Nucleotide-binding domain, leucine-rich repeat receptors (NLRs) mediate innate immunity by forming inflammasomes. Activation of the NLR protein NLRP1 requires autocleavage within its function-to-find domain (FIIND). In resting cells, the dipeptidyl peptidases DPP8 and DPP9 interact with the FIIND of NLRP1 and suppress spontaneous NLRP1 activation; however, the mechanisms through which this occurs remain unknown. Here we present structural and biochemical evidence that full-length rat NLRP1 (rNLRP1) and rat DPP9 (rDPP9) form a 2:1 complex that contains an autoinhibited rNLRP1 molecule and an active UPA–CARD fragment of rNLRP1.

Two-dimensional class averages showed that rDPP9 formed dimers, but only one subunit was bound to NLRP1 in most of the particles. We used the particles with one rDPP9 subunit bound by rNLRP1 for further cryo-EM analysis. After 3D classification, a subset of 182,116 particles was used for final 3D reconstruction, generating a map with a global resolution of 3.18 Å. Unexpectedly, the liganded rDPP9 subunit is bound by two rNLRP1 molecules, which we hereafter term the 2:1 rNLRP1–rDPP9 complex. The first rNLRP1 molecule contains the complete FIIND, which has a conformation nearly identical to that observed in the crystal structure of the free FIIND; the remaining domains of this rNLRP1 molecule are not discernible in the cryo-EM density. In the second rNLRP1 molecule, only the UPA domain is well defined. Three surfaces mediate the formation of the 2:1 rNLRP1–rDPP9 complex. The first surface is mediated by ZU5 of rNLRP1, which binds to one lateral side of the β-propeller domain of rDPP9 (termed the ZU5-binding site of rDPP9). The second interface is formed by the deep insertion of an N-terminal loop (N-loop) from the UPA domain of the second rNLRP1 molecule into the rDPP9 substrate-binding channel (termed the UPA-binding site) (blue box). The substrate-binding groove of rDPP9 is completely blocked by the UPA N-loop. Additionally, the homodimerization interface of the two UPA domains also contributes to formation of the 2:1 complex (termed the UPA dimerization site) (yellow box).

>MEESQSKQESNTRVAQHGSQQDVDPTFQTKRALEKERSKPRPRPLPRVQLQSLPGWSSTSKDVPLSQLIREMDHESRRCIHRSKKKLDRSEHISQGTIPEIYEKRKETISHTQSMEQKYLFQNFTKLLLLQKCCPGGSEKLVRESWHPCVPEEGGHMIEIQDLFDPNLDTEKKPQLVIIEGAAGIGKSTLARQVKRAWDEGQLYRDRFQHVFFFSCRELAQCKQLSLAELIAQGQEVPTAPTRQILSRPEKLLFILDGIDEPAWVLEDQNPELCVHWSQAQPVHTLLGSLLGKSILPEASLMLTARTTALQKLVPSLGQPHRVEVLGFSEFERKDYFYKYFAKERNTIIDFNLIGSIPVLLTLCEVPWVCWLLCTCLEKQMQQGEVLSLTSQTTTALCLKYLSLTIPGQHLSTQLRTLCSLAAEGICQRRTLFSKSDLCKQGLAEDAIATFLKIGVLQRQPSSLSYSFAHLCLQEFFAAMSYILEDSEEAHGDMGNDRTVETLVERYGRQNLFEAPTVRFLLGLLNTREMREMENIFACKFPWETKLKLLQSIIGEPFCQPCHLGLFHCLYENQEEELLTETMLCFPLTASGPNHMEATVFQTNVKRLVIQTDMELMVVTFCITFSHVRSLRLKGKGQQEYKLTAPAMVLYRWTPISEASWKVLFSNLKCTRNLEELDLSGNPLSYSAVRSLCTALRQPGCRLKTLWLVDCGLTSRCCSFLASMLSAHSRLAELDLRLNDLGDNGVRQLCEGLRNPACNLSILRLDQASLSEQVITELRALETKNPKLFISSTWMSHMTMPTENTDGEESLTSSKQQQQQSGDKHMEPLGTDDDFWGPSGPVSTEVVDRERNLYRVRLPMAGSYHCPSTGLHFVVTRAVTIEIGFCAWSQFLHETPLQHSHMVAGPLFDIKAEHGAVTAVCLPHFVSLQEGKVDSSLFHVAHFQDHGMVLETPARVEPHFAVLENPSFSPMGVLLRMIPAVGHFIPITSITLIYYRLYLEDITFHLYLVPNDCTIRKAIDEEELKFQFVRINKPPPVDALYVGSRYIVSSSKEVEILPKELELCYRSPRESQLFSEIYVGNIGSGINLQLTDKKYMNLIWEALLKPGDLRPALPRMASAPKDAPALLHFVDQHREQLVARVTSVDPLLDKLHGLVLSEEDYETVRAEATNQDKMRKLFRGSRSWSWDCKDHFYQALKETHPHLIMDLLEKSGGVSVRL[2x];>MSGGVSPVEQVAAGDMDDTAARFCVQKHSWDGLRNIIHGSRKSSGLIVSKAPHDFQFVQKPDESGPHSHRLYYLGMPYGSRENSLLYSEIPKKVRKEALLLLSWKQMLDHFQATPHHGVYSREEELLRERKRLGVFGITSYDFHSESGLFLFQASNSLFHCRDGGKNGFMVSPMKPLEIKTQCSGPRMDPKICPADPAFFSFINNNDLWVANIETGEERRLTFCHQGSASVLDNPKSAGVATFVIQEEFDRFTGCWWCPTASWEGSGGLKTLRILYEEVDESEVEVIHVPSPALEERKTDSYRYPRTGSKNPKIALKLAELQTDHQGKIVSSCEKELVQPFSSLFPKVEYIARAGWTRDGRYAWAMFLDRPQQRLQLVLLPPALFIPTLESEAQWQEAARAIPKNVQPFIIYEEVTNVWINVHDIFHPFPQAEGQQDFCFLRANECKTGFCHLYRVTVDLKTNDYDWTEPLSPAEDEFKCPIKEEVALTSGEWEVLSRHGSKIWVNEQTKLVYFQGTKDTPLEHHLYVVSYESAGEIVRLTTPGFSHSCSMSQNFDMFVSHYSSVSTPPCVHVYKLSGPDDDPLHKQPRFWASMMEAASCPPDYVPPEIFHFHTRADVQLYGMIYKPHTLQPGRKHPTVLFVYGGPQVQLVNNSFKGIKYLRLNTLASLGYAVVVIDGRGSCQRGLHFEGALKNQMGQVEIEDQVEGLQYVAEKYGFIDLSRVAIHGWSYGGFLSLMGLIHKPQVFKVAIAGAPVTVWMAYDTGYTERYMDVPENNQQGYEAGSVALHVEKLPNEPNRLLILHGFLDENVHFFHTNFLVSQLIRAGKPYQLQIYPNERHSIRCRESGEHYEVTLLHFLQEHL[2x]Currently, the abnormal activation of RAS-RAF-MEK1/2-ERK1/2 signaling cascade has been confirmed in more than 33% of tumors, and it is considered one of the most important drivers of malignant progression, invasion, and metastasis of tumors. ERK1/2 and ERK5 have certain homology (66%) and possess many common substrates, such as c-Myc, c-Fos, RSK, etc., thus participating in the regulation of the same cellular process. By utilizing the principle of polypharmacology, we computationally designed SKLB-D18, a first-in-class molecule that selectively targets ERK1/2 and ERK5, with nanomolar potency and high specificity for both targets. The co-crystal structures revealed that SKLB-D18 occupies the ATP-binding sites of both ERK2 and ERK5 simultaneously.

The co-crystal structure of SKLB-D18 with ERK5 revealed that SKLB-D18 also occupies the ATP-binding site of ERK5, while a significant bidentate hydrogen bond is established between the 2-aminopyrimidine moiety and Met140. Furthermore, the carbonyl of amide group establishes a hydrogen bond with Lys84, and the NH of amide group forms a water-mediated hydrogen bond with Asp200. Additionally, the morpholinyl and 3-((dimethylamino)methyl)phenyl group are oriented towards the solvent regions on either side, respectively. Structural analysis revealed that the SKLB-D18 in complex with ERK1/2 establishes a more extensive interaction network compared to its binding with ERK5, as evidenced by (1) additional hydrogen bonds at the binding interface, (2) enhanced hydrophobic complementarity, and (3) optimized electrostatic interactions. The bidentate hydrogen bonds formed between the 2-aminopyrimidine scaffold and ERK1/2/5 are crucial for the stable binding. SKLB-D18 exhibits nanomolar potency against ERK1/2 and ERK5 with half-maximal inhibitory concentration (IC50) values of 38.69 ± 0.62 nM, 40.12 ± 0.95 nM and 59.72 ± 1.21 nM, respectively. The isothermal titration calorimetry (ITC) assay further confirmed the binding affinity of SKLB-D18 to ERK1/2/5, with a dissociation constant (Kd) of 126.9 nM, 209.8 nM and 468.2 nM, respectively. SKLB-D18 dose-dependently inhibited p-ERK5, with the 50 mg/kg dose showing stronger inhibition than XMD8-92 and combination therapy groups.

>[2x]TFDVGDEYEIIETIGNGAYGVVSSRRRRLTGQQVAIKKIPNAFDVVTNAKRTLRELKILKHFKHDNIIAIKDILRPTVPYGEFKSVYVVLDLMESDLHQIIHSSQPLTLEHVRYFLYQLLRGLKYMHSAQVIHRDLKPSNLLVNENCELKIGDFGMARGLCTSPAEHQYFMTEYVATRWYRAPELMLSLHEYTQAIDLWSVGCIFGEMLARRQLFPGKNYVHQLQLIMMVLGTPSPAVIQAVGAERVRAYIQSLPPRQPVPWETVYPGADRQALSLLGRMLRFEPSARISAAAALRHPFLAKYHDPDDEPDCAPPFDFAFDREALTRERIKEAIVAEIEDFHARRE During chromosome replication, the nascent leading strand is synthesized by DNA polymerase epsilon (Pol ε), which associates with the sliding clamp processivity factor proliferating cell nuclear antigen (PCNA) to form a processive holoenzyme. For high-fidelity DNA synthesis, Pol ε relies on nucleotide selectivity and its proofreading ability to detect and excise a misincorporated nucleotide. For proofreading and mismatch excision, the 3′ end of the nascent strand must be partially melted from the template strand and guided toward the Pol ε exonuclease domain active site (exo site), which is located almost 40 Å away from the pol site. Our atomic model of human Pol ε cat closely resembles the crystal structure of the S. cerevisiae homolog, with an identical domain organization in the ‘right-hand’-shaped B-family DNA Pol fold consisting of an N-terminal domain (NTD) and the Palm, Exonuclease (Exo), Finger and Thumb domains.

The second intermediate (the Frayed Substrate state) displays a frayed nascent strand–template strand junction that is more reminiscent of the Mismatch Excision conformer, with the two terminal bases of the nascent strand unpaired from the template. In the Frayed Substrate state, we observe cryo-EM density at the junction of the template and nascent DNA strands that can accommodate two bases of single-stranded DNA of the nascent strand at the entry cavity of the Exo domain. The atomic model of the Frayed state shows how the terminal bases of the nascent strand are loosely held at the Exo domain near residues N363, F366, H422 and N423 and traject away from the template strand, from which they are physically separated by α-helix 3 of the Exo domain (‘wedge helix’) that obscures the direct path between the pol and exo sites. Despite being melted from the template strand and held at the surface of the Exo domain, the terminal erroneous base is still located more than 10 Å from the exo site in the Frayed state. The upstream portion of the dsDNA is released from its interactions at the tip of the Thumb domain (R1041 and Q1049 at nascent strand n-5 and n-6 and K1050 at template position n-9) and moves away from the Thumb and toward the P domain. In this configuration, the coordination of DNA at the P domain is more extensive than we observe in structures with matched DNA, with the backbone of the nascent strand held tightly against the positively charged surface of the P domain formed by residues R728, K733 and H735. This ‘handover’ of the DNA from the Thumb to the P domain could be initiated by the Thumb’s tilting DNA-binding surface during the transition toward the Arrest state, which the DNA compensates for through an in-plane tilt that brings the upstream region closer to the P domain. Positions n-3 and n-4 of the nascent strand remain coordinated by a flexible loop at positions 970–980 of the Thumb domain that harbors three positively charged residues K974, R975 and R976.

> MSLRSGGRRRADPGADGEASRDDGATSSVSALKRLERSQWTDKMDLRFGFERLKEPGEKTGWLINMHPTEILDEDKRLGSAVDYYFIQDDGSRFKVALPYKPYFYIATRKGCEREVSSFLSKKFQGKIAKVETVPKEDLDLPNHLVGLKRNYIRLSFHTVEDLVKVRKEISPAVKKNREQDHASDAYTALLSSVLQRGGVITDEEETSKKIADQLDNIVDMREYDVPYHIRLSIDLKIHVAHWYNVRYRGNAFPVEITRRDDLVERPDPVVLAFDIETTKLPLKFPDAETDQIMMISYMIDGQGYLITNREIVSEDIEDFEFTPKPEYEGPFCVFNEPDEAHLIQRWFEHVQETKPTIMVTYNGDFFDWPFVEARAAVHGLSMQQEIGFQKDSQGEYKAPQCIHMDCLRWVKRDSYLPVGSHNLKAAAKAKLGYDPVELDPEDMCRMATEQPQTLATYSVSDAVATYYLYMKYVHPFIFALCTIIPMEPDEVLRKGSGTLCEALLMVQAFHANIIFPNKQEQEFNKLTDDGHVLDSETYVGGHVEALESGVFRSDIPCRFRMNPAAFDFLLQRVEKTLRHALEEEEKVPVEQVTNFEEVCDEIKSKLASLKDVPSRIECPLIYHLDVGAMYPNIILTNRLQPSAMVDEATCAACDFNKPGANCQRKMAWQWRGEFMPASRSEYHRIQHQLESEKFPPLFPEGPARAFHELSREEQAKYEKRRLADYCRKAYKKIHITKVEERLTTICQRENSFYVDTVRAFRDRRYEFKGLHKVWKKKLSAAVEVGDAAEVKRCKNMEVLYDSLQLAHKCILNSFYGYVMRKGARWYSMEMAGIVCFTGANIITQARELIEQIGRPLELDTDGIWCVLPNSFPENFVFKTTNVKKPKVTISYPGAMLNIMVKEGFTNDQYQELAEPSSLTYVTRSENSIFFEVDGPYLAMILPASKEEGKKLKKRYAVFNEDGSLAELKGFEVKRRGELQLIKIFQSSVFEAFLKGSTLEEVYGSVAKVADYWLDVLYSKAANMPDSELFELISENRSMSRKLEDYGEQKSTSISTAKRLAEFLGDQMVKDAGLSCRYIISRKPEGSPVTERAIPLAIFQAEPTVRKHFLRKWLKSSSLQDFDIRAILDWDYYIERLGSAIQKIITIPAALQQVKNPVPRVKHPDWLHKKLLEKNDVYKQKKISELFTLEGRRQVTMAEA>MGGHHHHHHGGQEKDASSQGFLPHFQHFATQAIHVGQDPEQWTSRAVVPPISLSTTFKQGAPGQHSGFIYSRLGNPTRNCLEKAVAALDGAKYCLAFASGMAATVTITHLLKAGDQIICMDDVYGGTNAYFRQVASEFGLKISFVDCSKIKLLEAAITPETKLVWIETPTNPTQKVIDIEGCAHIVHKHGDIILVVDNTFMSPYFQRPLALGADISMYSATKYMNGHSDVVMGLVSVNCESLHNRLRFLQNSLGAVPSPIDCYLCNRGLKTLHVRMERHFKNGMAVAQFLESNPWVEKVIYPGLPSHPQHELVKRQCTGCGGMVTFYIKGTLQHAEIFLKNLKLFTLAVSLGGFESLAELPASMTHASVLKNDRD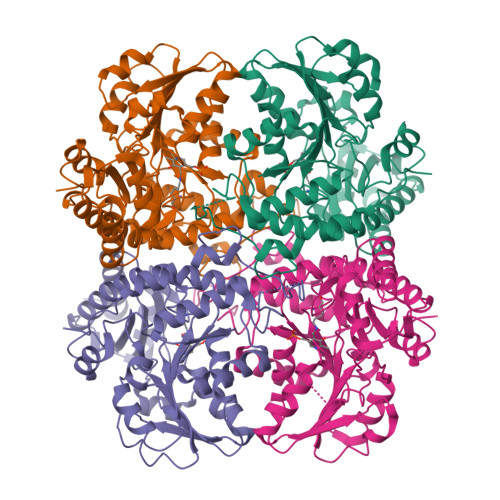VLGISDTLIRLSVGLEDEEDLLEDLDQALKAAHPPSGSHS[8x]>MPLVSMKDM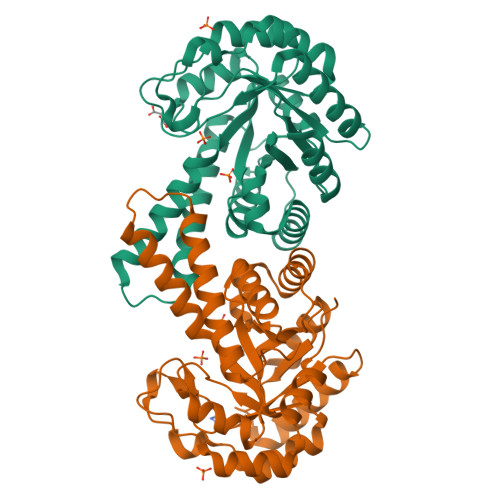LNHGKENGYAVGQFNINNLEFGQAILQAAEEEKSPVIIGVSVGAANYMGGFKLIVDMVKSSMDSYNVTVPVAIHLDHGPSLEKCVQAIHAGFTSVMIDGSHLPLEENIELTKRVVEIAHSVGVSVEAELGRIGGQEDDVVAESFYAIPSECEQLVRETGVDCFAPALGSVHGPYKGEPKLGFDRMEEIMKLTGVPLVLHGGTGIPTKDIQKAISLGTAKINVNTESQIAATKAVREVLNNDAKLFDPRKFLAPAREAIKETIKGKMREFGSSGKA[2x]> HHHHHHMKLLENSSFEAINSQLTVETGDAHIIGRIESY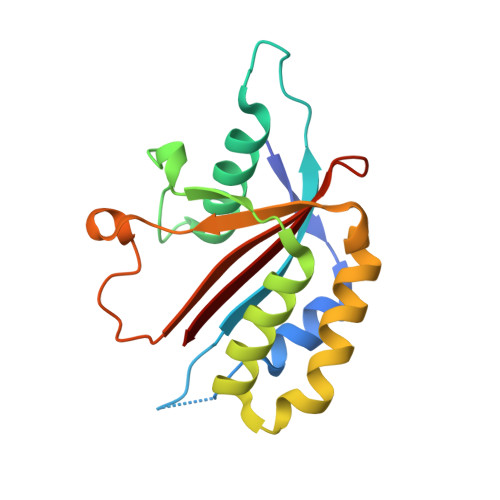SCKPLSDKCSRKTLFYLIATLNESFRPDYDFSTARSHEFSREPSLSWVVNAVNCSLFSAVREDFKDLKPQLWNAVDEEICLAECDIYSYNPDLDSDPFGEDGSLWSFNYFFYNKRLKRIVFFSCRS> SMSLELQEHCSLKPYNTFGIDVRARLLAHARDEADVREALALARERGLPLLVIGGGSNLLLTRDVEALVLRMASQGRRIVSDAADSVLVEAEAGEAWDPFVQWSLERGLAGLENLSLIPGTVGAAPMQNIGAYGVELKDVFDSLTALDRQDGTLREFDRQACRFGYRDSLFKQEPDRWLILRVRLRLTRRERLHLDYGPVRQRLEEEGIASPTARDVSRVICAIRREKLPDPAVLGNAGSFFKNPLVDATQAERLRQAFPDLVGYPQADGRLKLAAGWLIDKGGWKGFRDGPVGVHAQQALVLVNHGGATGAQVRALAERIQEDVRRRFGVELEPEPNLY

The resulting UDP-N-acetylglucosamine enolpyruvate (UNAGEP) is reduced by the UNAGEP reductase, MurB, to generate UNAM. All MurB proteins known to date are monomeric flavoenzymes that bind strongly a stoichiometric amount of flavin adenine dinucleotide (FAD). The catalytic cycle can be divided into two half reactions and follows the scheme of a ping-pong bi bi mechanism. Here, we present the crystal structure of NADP+-bound PaMurB, which establishes the co-localization of the NADPH and UNAGEP binding sites and supports a ping pong reaction mechanism with sequential substrate binding.

Crystal form A belongs to the space group C2 with four molecules per asymmetric unit, while crystal form B belongs to P61 with one molecule per asymmetric unit; the solutions are in agreement with solvent content analysis by using Matthews coefficient. The two crystal structures are identical in protein and ligand conformations, except three loops involved in crystal contacts on one side of the protein (β6-β7, β12-α5 and α5-α6) with an overall root-mean-squared difference, rmsd, of 0.8 Å, based on 336 Cα atoms. In the following results and figures are based on crystal form B unless otherwise noted. Ala-83, located on the β6-β7 turn, is a Ramachandran plot outlier in crystal form B with well-defined electron density, possibly because of crystal contacts. In the substrate binding cleft in domain III strong continuous electron density was observed that corresponds well to a bound NADP+ molecule. The nicotinamide amide group is located on the si face of the isoalloxazine ring of FAD, and forms hydrogen bonds with the conserved Ser-239 and Glu-335 residues. The two rings are nearly parallel and juxtaposed together, with the nicotinamide C4n atom in close proximity to the isoalloxazine N5 atom (3.1 Å and 2.8 Å in crystal forms A and B, respectively). This suggests that the nicotinamide group is in a position that favors the first half-reaction. Crystal form B also shows electron density at this position, but refinement suggests that this site is occupied by a water molecule or a metal ion at lower occupancy. Potassium binding apparent in only crystal form A could be due to the five times higher potassium concentration in the crystallization liquor for form A compared to form B crystals.>[2x]GPGSMTTPNFELYGYFRSSCSGRLRIAFHLKSIPYTRHPVNLLKGEQHSDTYKSLNPTNTVPLLVVSNINNTVSPSSASFSIGQSLAALEY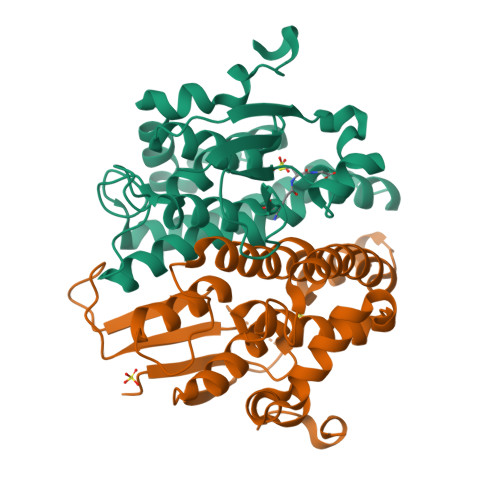LEEALPTNARPLLPPISNPVARAHVRTICNIIACDVQPVTNLKIQKKVKALDGDPTVWSRDLATQGFGAVEKLLELSAGRFCVGDEITLADVCLVPAVWAAERVGMDLARFPITKRVFEEMLKEEAVQKAHWQKQEDTPEDLRA>[2x]EHSEMKMSDMHSSASSQEYMAGMKNMHEKMMAAVNES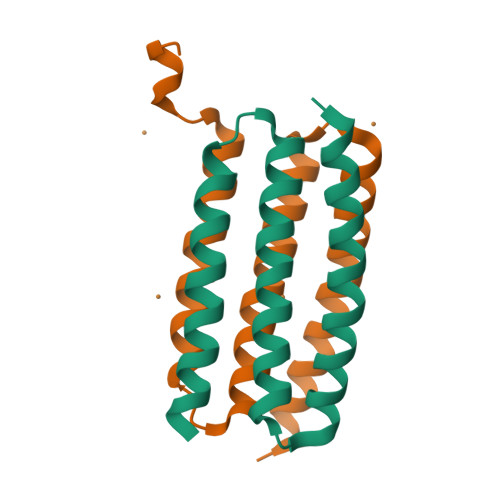NPDKAFAKGMIAHHEGAIAMAETELKYGKDPEMRKLAQDIIKAQKGEIEQMNKWLDSHK> RIYKIGTKALPCSECHDVFDCTGCLFEEKESSHVIPLKLNKKNPNDHKKLQKHHESLKLGDVKYYVNRGEGISGSLGTSSGNTLDDMDLINEEINKKRTNAQLDEKNFLENKNATVEQTKENIFLVPLKHLRDSQFVGELLVGTPPQTVYPIFDTGSTNVWVVTTACEEESCKKVRRYDPNKSKTFRRSFIEKNLHIVFGSGSISGSVGTDTFMLGKHLVRNQTF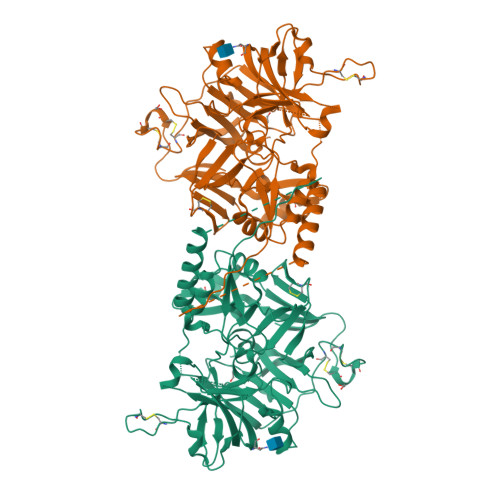GLVESESNNNKNGGDNIFDYISFEGIVGLGFPGMLSAGNIPFFDNLLKQNPNVDPQFSFYISPYDGKSTLIIGGISKSFYEGDIYMLPVLKESYWEVKLDELYIGKERICCDEESYVIFDTGTSYNTMPSSQMKTFLNLIHSTACTEQNYKDILKSYPIIKYVFGELIIELHPEEYMILNDDVCMPAYMQIDVPSERNHAYLLGSLSFMRNFFTVFVRGTESRPSMVGVARAKSKNENLYFQ> RVKRTYEVTRQNDNAVRIEPSSLGEEEDKEAKDKNSALQLKRSRYDPNKVFSNTNQGPEKNNLKGEQLGSQKKSSKYDEKITSNNELTTKKGLLGDSENETKYASSNSKFNVEVTHKIKNAKEIDKINRQRMWEEQQLRNAMAGQSDHPDDITLEGSDKYDYVFDTDAMIDYTNEEDDLLPEEKLQYEARLAQALETEEKRILTIQEARKLLPVHQYKDELLQEIKKNQVLIIMGETGSGKTTQLPQYLVEDGFTDQGKLQIAITQPRRVAATSVAARVADEMNVVLGKEVGYQIRFEDKTTPNKTVLKYMTDGMLLREFLTDSKLSKYSCIMIDEAHERTLATDILIGLLKDILPQRPTLKLLISSATMNAKKFSEFFDNCPIFNVPGRRYPVDIHYTLQPEANYIHAAITTIFQIHTTQSLPGDILVFLTGQEEIERTKTKLEEIMSKLGSRTKQMIITPIYANLPQEQQLKIFQ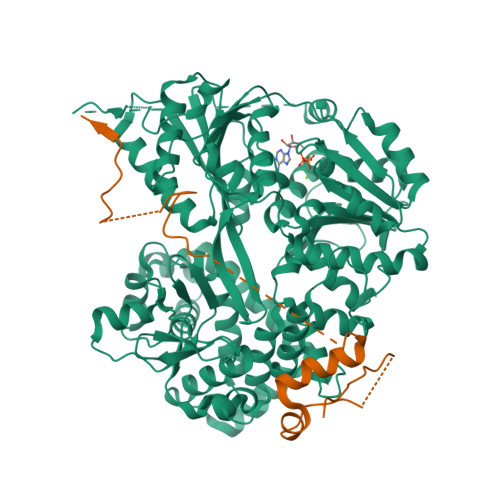PTPENCRKVVLATNIAETSLTIDGIRYVIDPGFVKENSYVPSTGMTQLLTVPCSRASVDQRAGRAGRVGPGKCFRIFTKWSYLHELELMPKPEITRTNLSNTVLLLLSLGVTDLIKFPLMDKPSIPTLRKSLENLYILGALNSKGTITRLGKMMCEFPCEPEFAKVLYTAATHEQCQGVLEECLTIVSMLHETPSLFIGQKRDAAASVLSEVESDHILYLEIFNQWRNSKFSRSWCQDHKIQFKTMLRVRNIRNQLFRCSEKVGLVEKNDQARMKIGNIAGYINARITRCFISGFPMNIVQLGPTGYQTMGRSSGGLNVSVHPTSILFVNHKEKAQRPSKYVLYQQLMLTSKEFIRDCLVIPKEEWLIDMVPQIFKDLI;> MSKFSLKLGSKTLKKNISKKTKKKNSLQKANLFDWDDAETASLSHKPQSKIKIQSIDKFDLDEESSSKKKLVIKLSENADTKKNDAPLVEYVTEKEYNEVPVEEFGDALLRGMGWESDSEQDSKGDKTQSRNKDVSNVSQIHPDGLGIGAKLNKAINVEEASFMPVVKIDKITGTKVDDDKKNKS>MGKIGIFFGTDSGNAEAIAEKISKAIGNAEVVDVAKASKEQFNSFTKVILVAPTAGAGDLQTDWEDFL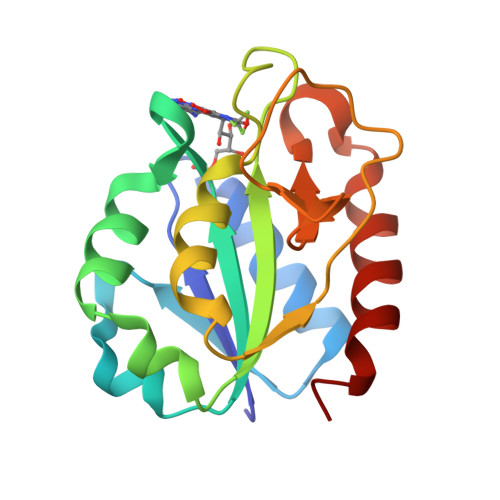GTLEASDFANKTIGLVGLGDQDTYSETFAEGIFHIYEKAKAGKVVGQTSTDGYHFEASKAVEGGKFVGLVIDEDNQDDLTDERISKWVEQVRGSFA[2x]>MKVLRHGLFKDRRVFDENYIPPELRVRRGEAEALARIYLNRLLSGAGLSDVNMIYGSIGRVGIGKTTLAKFTVKRVSEAAAKEGLTVKQAYVNAFNAPNLYTILSLIVRQTGYPIQVRGAPALDILKALVDNLYVENHYLLVILDEFQSMLSSPRIAAEDLYTLLRVHEEIPSRDGVNRIGFLLVASDVRALSYMREKIPQVESQIGFKLHLPAYKSRELYTILEQRAELGLRDTVWEPRHLELISDVYGEDKGGDGSARRAIV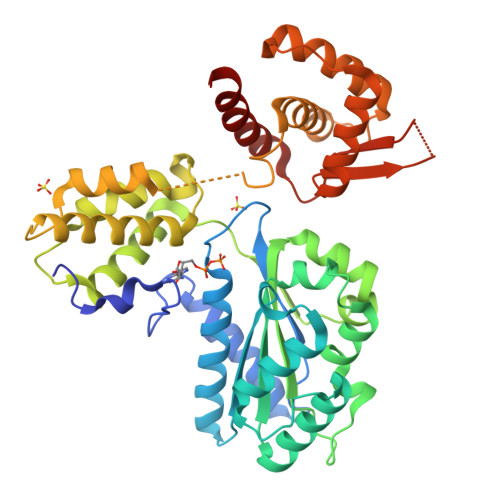ALKMACEMAEAMGRDSLSEDLVRKAVSENEAASIQTHELEALSIHELIILRLIAEATLGGMEWINAGLLRQRYEDASLTMYNVKPRGYTQYHIYLKHLTSLGLVDAKPSGRGMRGRTTLFRLAPHLPADRLIEVVDNIIQAKMASGYE[2x]> SNAPLKEQKVINTANIKTNSKLDLAEYENGLINIATQQFDTESHVLQLNQYIPEKLIDELVAKVEAPVLTNIIEQDYFGKQNSNELSLSGVMIGLAMSSSVSNEEAMSKGTEVAKQLIEAINKNDKYNKSPITFAIFKQESTSSLKNGTYI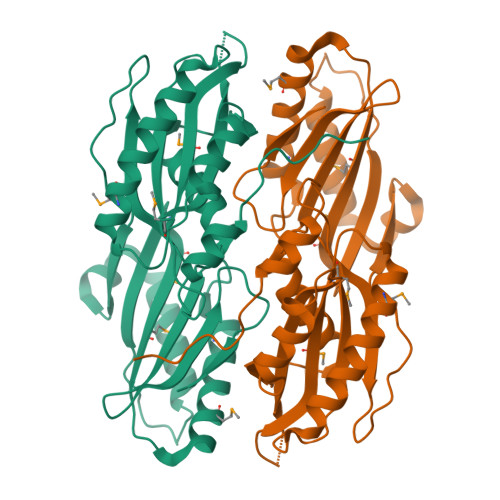ASATVQKNDTNLGNWSTIDEKSYSYPSDEFTQAHGEDNTKINNFAKEIKGFSNGDFIPVNAKVSYKKDQMDTLNMNIVIKYNGKTELMALTQLAAQGMLDKLPKDAKVQLQIKSESKIEAVIIKEKNSDKPFVSFL>MGHHHHHHHHHHMQSSVNEFLTPRHIDVQVVSQTRAKITLEPLERGFGHTLGNALRRILLSSMPGCAVVEAEIDGVLHEYSAIEGVQEDVIEILLNLKGLAIKLHGRDEVTLTLAKKGSGVVTAADIQLDHDVEIINGDHVIANLADNGALNMKLKVARGRGYEPADARQSDEDESRSIGRLQLDASFSPVRRVSYVVENARVEQRTNLDKLVLDLETNGTLDPEEAIRRAATILQQQLAAFVDLKGDSEPVVEEQEDEIDPILLRPVDDLELTVRSANCLKAENIYYIGDLIQRTEVELLKTPNLGKKSLTEIKDVLASRGLSLGMRLDNWPPASLKKDDKATA[2x];> MGMAYSYTEKKRIRKDFSKLPDVMDVPYLLAIQLDSYREFLQAGATKEQFRDVGLHAAFKSVFPIISYSGNAALEYVGYRLGEPAFDVKECVLRGVTFAVPLRVKVRLIIFDRESSNKAIKDIKEQEVYMGEIPLMTENGTFIINGTERVIVSQLHRSPGVFFDHDRGKTHSSGKLLYSARIIPYRGSWLDFEFDPKDCVFVRIDRRRKLPASVLLRALGYSTEEILNAFYATNVFHIKGETLNLELVPQRLRGEVASIDIKDGSGKVIVEQGRRITARHINQLEKAGVSQLEVPFDYLIGRTIAKAIVHPATGEIIAECNTELTLDLLAKVAKAQVVRIETLYTNDIDCGPFISDTLKIDNTSNQLEALVEIYRMMRPGEPPTKEAAETLFGNLFFSAERYDLSAVGRMKFNRRIGRTEIEGPGVLSKEDIIDVLKTLVDIRNGKGIVDDIDHLGNRRVRCVGEMAENQFRVGLVRVERAVKERLSMAESEGLMPQDLINAKPVAAAIKEFFGSSQLSQFMDQNNPLSEITHKRRVSALGPGGLTRERAGFEVRDVHPTHYGRVCPIETPEGPNIGLINSLATYARTNKYGFLESPYRVVKDSLVTDEIVFLSAIEEADHVIAQASATLNEKGQLVDELVAVRHLNEFTVKAPEDVTLMDVSPKQVVSVAASLIPFLEHDDANRALMGSNMQRQAVPTLRADKPLVGTGMERNVARDSGVCVVARRGGVIDSVDASRVVVRVADDEVETGEAGVDIYNLTKYTRSNQNTCINQRPLVSKGDVVARGDILADGPSTDMGELALGQNMRVAFMPWNGFNFEDSICLSERVVQEDRFTTIHIQELTCVARDTKLGPEEITADIPNVGEAALNKLDEAGIVYVGAEVQAGDILVGKVTPKGETQLTPEEKLLRAIFGEKASDVKDTSLRVPTGTKGTVIDVQVFTRDGVERDSRALSIEKMQLDQIRKDLNEEFRIVEGATFERLRAALVGAKAEGGPALKKGTEITDDYLDGLERGQWFKLRMADDALNEQLEKAQAYISDRRQLLDDKFEDKKRKLQQGDDLAPGVLKIVKVYLAIKRRIQPGDKMAGRHGNKGVVSVIMPVEDMPHDANGTPVDIVLNPLGVPSRMNVGQILETHLGLAAKGLGEKINRMLEEQRKVAELRKFLHEIYNEIGGREENLDELGDNEILALAKNLRGGVPMATPVFDGAKEREIKAMLKLADLPESGQMRLFDGRTGNQFERPTTVGYMYMLKLNHLVDDKMHARSTGSYSLVTQQPLGGKAQFGGQRFGEMEVWALEAYGAAYTLQEMLTVKSDDVNGRTKMYKNIVDGDHRMEAGMPESFNVLIKEIRSLGIDIELETE;> MLKDLLNLLKNQGQIEEFDAIRIGLASPEMIRSWSFGEVKKPETINYRTFKPERDGLFCAKIFGPVKDYECLCGKYKRLKHRGVICEKCGVEVALAKVRRERMGHIELASPVAHIWFLKSLPSRIGLLLDMTLRDIERVLYFESYVVIDPGMTTLEKGQLLNDEQYFEALEEFGDDFDARMGAEAVHELLNAIDLEHEIGRLREEIPQTNSETKIKKLSKRLKLMEAFQGSGNKPEWMVLTVLPVLPPDLRPLVPLDGGRFATSDLNDLYRRVINRNNRLKRLLDLAAPDIIVRNEKRMLQEAVDALLDNGRRGRAITGSNKRPLKSLADMIKGKQGRFRQNLLGKRVDYSGRSVITVGPTLRLHQCGLPKKMALELFKPFIFGKLEGRGMATTIKAAKKMVERELPEVWDVLAEVIREHPVLLNRAPTLHRLGIQAFEPVLIEGKAIQLHPLVCAAYNADFDGDQMAVHVPLTLEAQLEARALMMSTNNILSPANGEPIIVPSQDVVMGLYYMTREAINAKGEGMAFADLQEVDRAYRSGQASLHARVKVRINEKIKGEDGQLTANTRIVDTTVGRALLFQVVPAGLPFDVVNQSMKKKAISKLINHCYRVVGLKDTVIFADQLMYTGFAYSTISGVSIGVNDFVIPDEKARIINAATDEVKEIESQYASGLVTQGEKYNKVIDLWSKANDEVSKAMMANLSKEKVVDREGKEVDQESFNSMYMMADSGARGSAAQIRQLAGMRGLMAKPDGSIIETPITANFREGLNVLQYFISTHGARKGLADTALKTANSGYLTRRLVDVAQDLVVTEIDCGTEHGLLMSPHIEGGDVVEPLGERVLGRVIARDVFKPGSDEVIVPAGTLIDEKWVDFLEVMSVDEVVVRSPITCETRHGICAMCYGRDLARGHRVNIGEAVGVIAAQSIGEPGTQLTMRTFHIGGAASRTSAADNVQVKNGGTIRLHNLKHVVRADGALVAVSRSGELAVADDFGRERERYKLPYGAVISVKEGDKVDPGAIVAKWDPHTHPIVTEVDGTVAFVGMEEGITVKRQTDELTGLTNIEVMDPKDRPAAGKDIRPAVKLIDAAGKDLLLPGTDVPAQYFLPANALVNLTDGAKVSIGDVVARIPQETSKTRDITGGLPRVADLFEARRPKEPSILAEISGTISFGKETKGKRRLVITPNDGSDPYEELIPKWRHLNVFEGEQVNRGEVISDGPSNPHDILRLLGVSSLAKYIVNEIQDVYRLQGVKINDKHIETILRQMLRKVEVSESGDSSFIKGDQVELTQVLEENEQLGTEDKFPAKYERVLLGITKASLSTESFISAASFQETTRVLTEAAVTGKRDFLRGLKENVVVGRLIPAGTGLAYHSERKRQRDLGKPQRVSASEAEAALTEALNSSGNGSGSWSHPQFEK;> MARVTVEDCLDNVDNRFELVMLATKRARQLATGGKEPKVAWENDKPTVVALREIASGLVDENVVQQEDIVEDEPLFAAFDDEANTEAL;> MALKKEGPEFDHDDEVLLLEPGIMLDESSADEQPSPRATPKATTSFSSKQHKHIDYTRALDATQLYLNEIGFSPLLTPEEEVHFARLAQKGDPAGRKRMIESNLRLVVKIARRYVNRGLSLLDLIEEGNLGLIRAVEKFDPERGFRFSTYATWWIRQTIERAIMNQTRTIRLPIHVVKELNVYLRAARELTHKLDHEPSPEEIANLLEKPVAEVKRMLGLNERVTSVDVSLGPDSDKTLLDTLTDDRPTDPCELLQDDDLSESIDQWLTELTDKQREVVIRRFGLRGHESSTLEEVGQEIGLTRERVRQIQVEALKRLREILEKNGLSSDALFQLEHHHHHH;> GAMGMSEEELEQDELDGADEDDGEELAAADDGEADSGDGDEAPAPGKKAKAAVVEEELPSVEAKQKERDALAKAMEEFLSRGGKVQEIEPNVVADPPKKPDSKYGSRPI

Pseudomonas aeruginosa (Pae) SutA adapts bacteria to hypoxia and nutrition-limited environment during chronic infection by increasing transcription activity of an RNA polymerase (RNAP) holoenzyme comprising the stress-responsive σ factor σS (RNAP-σS). To understand the molecular mechanism of SutA activation, here we determined cryo-EM structures of RNAP-σS holoenzyme at 4.1 Å, SutA-bound RNAP-σS holoenzyme at 3.1 Å (SutA-RNAP-σS, open lobe) and 3.9 Å (SutA-RNAP-σS, closed lobe), and SutA-bound RNAP-σS promoter open complex (SutA-σS-RPo) at 5.8 Å. The structures reveal that SutA pinches RNAP-β protrusion with its RNAP-binding domain and wedges RNAP-β lobe open to facilitate promoter unwinding with its wedge loop and N-terminal D/E-rich region. SutA anchors RNAP-β protrusion through its RBD and wedges open β lobe through its wedge loop to facilitate RPo formation.

To better understand the action of SutA upon RPo formation, we incubated SutA-RNAP-σS with a duplex rrn promoter DNA (−49 to +21) for 20 s and immediately applied the reaction mixture on grids for cryo-EM data collection. However, we only obtained one major 3D class of single particles, from which a cryo-EM map at 5.8 Å resolution of SutA-bound RPo (SutA-σS-RPo) was reconstructed. The map shows clear density for upstream promoter dsDNA (−35 to −12), 14 bp downstream dsDNA (+4 to +17), and the −10 element (−11 to −10) of non-template ssDNA of the transcription bubble. The cryo-EM map also shows clear signals for SutA-RBD that interacts with RNAP-β protrusion as in the structure of SutA-RNAP-σS (open lobe), but no signal for SutA wedge loop, SutA-NTD, and SutA-CTD, indicating that SutA-RBD remains bound to RNAP upon RPo formation. Structure superimposition of SutA-σS-RPo and SutA-RNAP-σS structures suggests that formation of RPo closes both the β’ clamp and β lobe of RNAP. SutA wedge loop opens the main cleft and facilitate the rrn promoter loading and unwinding. Loading of promoter DNA likely displaces SutA-NTD in the main cleft, disengages the wedge loop, and resumes the flexibility of lobe domain necessary for subsequent promoter unwinding steps.>GPLGSARRLYVGNIPFGITEEAMMDFFNAQMRLGGLTQAPGNPVLAVQINQDKNFAFLEFRSVDETTQAMAFDGIIF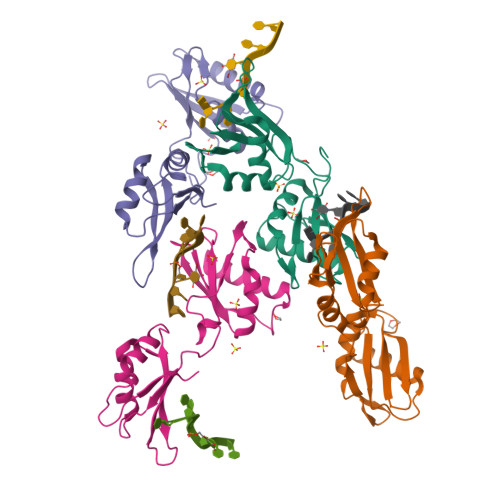QGQSLKIRRPHDYQPLPGAHKLFIGGLPNYLNDDQVKELLTSFGPLKAFNLVKDSATGLSKGYAFCEYVDINVTDQAIAGLNGMQLGDKKLLVQRAS[4x]The FfIBP from Flavobacterium frigoris PS1 exhibits high TH activity and relatively strong recrystallization inhibition activity. The FfIBP structure is composed of parallel β-strands in a helical pattern, which is mainly stabilized by inner hydrophobic interactions and intramolecular hydrogen bonds with long α415. Additionally, the FfIBP has a capping head region that consists of two small turns and β-strands, which contain a disulfide bond. This disulfide bond increases the overall rigidity of the protein and reduces residual movement at the ice-binding site, thereby augmenting TH activity and protein stability.

Based on the CD and MD simulation data, four mutants annotated as FfIBP_CC1 (A101C-A120C), FfIBP_CC2 (S96C-L132C), FfIBP_CC3 (M249C-N270C), and FfIBP_CC4 (G160C-S176C), possibly forming disulfide bonds, were generated. Finally, the most flexible region identified by MD simulation was selected as the 4th disulfide mutant (FfIBP_CC4). To confirm the disulfide formation, we solved the crystal structures of the FfIBP_CC1, CC2, CC3, and CC4 at 2.0, 2.1, 2.0, and 2.0 Å, respectively. Among these mutants, only FfIBP_CC1 and FfIBP_CC4 formed disulfide bonds within the intended area. When the RMSD values of alpha carbon mutants were compared with the wildtype, relatively high RMSD values exceeding 0.4 Å were observed around the mutation sites of FfIBP_CC2, FfIBP_CC3, and FfIBP_CC4. Unexpectedly, in the case of FfIBP_CC4, the Tm decreased by − 5 °C, possibly due to conformational distortion caused by disulfide bond formation and a decrease in protein stability. However, we postulate that the forced angle change due to the disulfide bond negatively affects neighboring residues involved in the hydrophobic core, such as Trp174, Leu178, and Val198. It is worth noting that the initial 350 nm/330 nm ratio for FfIBP_CC4 is lower than that of other mutants, including the wild-type.

> HMSLSVANSTYETTALNSQKSSTDQPNSGSKSGQTLDLVNLGVAANFAILSKTGITDVYKSAITGDVGASPITGAAILLKCDEVTGTIFSVDAAGPACKITDASRLTTAVGDMQIAYDNAAGRLNPDFLNLGACTIGGKTLTPGLYKWTCTLNIPTDITISGSSTDVWIFQVAGNLNMSSAVRITLAGGAQAKNIFWQTAGAVTLGSTSHFEGNILSQTGINMKTAASINGRMMAQTAVTLQMNTVTIPQ>MTRNQLHNWLNAGFFGLLLLLIHVQGQDSPEANPIRNTHTGQIQGSLIHVKDTKAGVHTFLGIPFAKPPVGPLRFAPPEAPEPWSGVRDGTAHPAMCLQNLDMLNEAGLPDMKMMLSSFPMSEDCLYLNIYTPAHAHEGSNLPVMVWIHGGALVIGMASMFDGSLLTVNEDLVVVTIQYRLGVLGFFSTGDQHARGNWGYLDQAAALRWVQQNIAHFGGNPDRVTIFGESAGGTSVSSHVVSPMSQGLFHGAIMESGVALLPDLISETSEMVSTTVAKLSGCEAMDSQALVRCLRGKSEAEILAINKVFKMIPAVVDGEFFPRHPKELLASEDFHPVPSIIGVNNDEFGWSIPVVMGSAQMIKGITRENLQAVLKDTAVQMMLPPECSDLLMEEYMGDTEDAQTLQIQFTEMMGDFMFVIPALQVAHFQRSHAPVYFYEFQHPPSYFKDVRPPHVKADHADEIPFVFASFFWGMKLDFTEEEELLSRRMMKYWANFARHGNPNSEGLPYWPVMDHDEQYLQLDIQPAVGRALKAGRLQFWTKTLPQKIQELKASQDKHREL[4x]

Mouse Ces2c (mCes2c) is suggested as potential ortholog of human CES2. Similarly, in a murine colitis model and in obese mice, a decline of mCes2 expression is observed in the colon. Both enzymes, hCES2 and mCes2c, can hydrolyze classical carboxylesterase substrates including acyl-carnitine, they can be inhibited by anti-rat CES antibodies, and they have high activities towards triacylglycerols, diacylglycerols, and monoacylglycerols as substrate. The monomeric unit of mCes2c harbors an α/β-hydrolase fold with additional modules and insertions. The core of the α/β-hydrolase domain in mCes2c is built by amino acids V57-M96, L126-L260, D317-G349, and F418-N501, and it contains the active site residues S230, E347, and H459 forming a catalytic triad.

Here, we present the first crystal structure of mCes2c to 2.12 Å resolution. The structure contains four monomers in the asymmetric unit (pairwise RMSD values of 0.15 Å), which are referred to as chains A–D, with the biological assembly being a monomer. In all 4 chains, residues C97-C125 and C282-C293 form disulfide bonds. In each monomer of the experimental structure of mCes2c, additional electron density was observed that could ideally be fitted to one molecule of nicotinamide (NCA) in the substrate binding pockets with 100% occupancy. Analysis of the ligand–protein interaction reveals H-bonding of the NCA-carbonyl oxygen to the backbone amide protons of oxyanion-hole residues G151, A152, and A231. The presence of NCA leads to restricted access to the active site within the core. In the structure we found electron density at the Z-site and could fit a single NCA molecule in chains A and B. Only residual electron density can be observed in chains C and D, which could not be fitted unambiguously to a distinct small molecule with full occupancy. In mCes2c, the entrance to the substrate binding pocket of each monomer is framed mostly by flexible loops and helical parts of the cap, the RD including the gate residue M417, and parts of the core. Similar to the product release mechanism of hCES1 proposed by Bencharit et al. next to the active site in the site door region, mCes2c harbors the conserved gate (M417) and switch (F418) residues. The low-resolution shape of mCes2c reconstructed from SAXS profiles fit (ꭓ2 = 1.4) to the experimentally determined crystal structure of mCes2c. Together the biochemical, structural, and biophysical experiments all corroborate the predominantly monomeric state of mCes2c.> QDASTKKLSECLRRIGDELDSNMELQ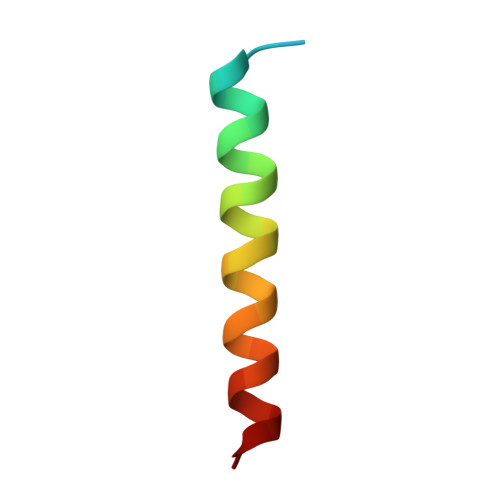RMIAD Recently, the 4.1 protein, ezrin, radixin and moesin (FERM)-domain–containing kindlin family of proteins has emerged as key players involved in integrin activation. Kindlins cooperate with talin to positively regulate integrin activation. Talin binds the membrane proximal NPxY motif, whereas kindlin binds the membrane distal NxxY motif. Here, we report the crystal structure of human full-length kindlin-3.

Unexpectedly, we observed 3 molecules of kindlin-3 forming a homotrimer in an asymmetric unit of the crystal with each protomer dovetailing the next. Kindlin-3 trimer adopts a triangular prism-like structure along the noncrystallographic 3-fold symmetry axis with the following dimensions: an outer-side length of approximately 110 Å, an inner cavity width of approximately 60 Å, and a height of approximately 90 Å. Each kindlin-3 monomer adopts a cloverleaf-like overall conformation. The F1 domain resides at the center of the kindlin-3 structure with the F1 loop wrapped around its α/β barrel and interacting with other domains. The crystal structure of kindlin-3 trimer also reveals that the additional α2PH helix in the PH domain of protomer A directly wedges into a cleft involving the 2 C-terminal helices (α1F3 and α2F3) and the β-sheet (β5F3-β7F3) in the F3 domain of protomer B, thereby forming extensive contacts. The residues Thr467, Ser468, Val470, Gln471, Ala475, and Ser478 in α2PH of protomer A interact with Ser595, Gln599, Trp600, Ser642, Thr643, Leu656, and Gln659 located in β5F3′ and its preceding loop, and α1F3′ of F3 domain in protomer B (the prime ′ refers to protomer B in the trimer), respectively. In addition, the C-terminus of α1PH and its subsequent loop in the PH domain pack against the 2 C-terminal helices and their connecting loop in the F3 domain of protomer B, through H-bonding (Gln443 in protomer A with main chain of Phe640 in protomer B) and salt bridge (Arg447 in A-Asp653 in B) interactions. In the kindlin-3 trimer, the F3-integrin-binding site in each protomer is occluded by the α2PH helix of the PH domain from the neighboring protomer, suggesting that trimer formation could inhibit kindlin-3 binding to integrin β cytoplasmic tails. Although kindlin-3 monomer binds, albeit weakly with the dissociation constant (Kd) of approximately 200 μM, with integrin β1 cytoplasmic tail, kindlin-3 trimer does not show any detectable binding. Therefore, we proposed that the triple mutations Q471A, A475F, and S478A (henceforth referred to as AFA) could disrupt the protomer–protomer interface in kindlin-3 trimer.

>MAGMKTASGDYIDSSWELRVFVGEEDPEAESVTLRVTGESHIGGVLLKIVEQINRKQDWSDHAIWWEQKRQWLLQTHWTLDKYGILADARLFFGPQHRPVILRLPNRRALRLRASFSQPLFQAVAAICRLLSIRHPEELSLLRAPEKKEKKKKEKEPEEELYDLSKVVLAGGVAPALFRGMPAHFSDSAQTEACYHMLSRPQPPPDPLLLQRLPRPSSLSDKTQLHSRWLDSSRCLMQQGIKAGDALWLRFKYYSFFDLDPKTDPVRLTQLYEQARWDLLLEEIDCTEEEMMVFAALQYHINKLSQSGXXXXXXXXXXXXXXXXXXXXXXXXXXXXXXXXXXXXXXXXXPELKDHLRIFRIPRRPRKLTLKGYRQHWVVFKETTLSYYKSQDEAPGDPIQQLNLKGCEVVPDVNVSGQKFCIKLLVPSPEGMSEIYLRCQDEQQYARWMAGCRLASKGRTMADSSYTSEVQAILAFLSLQRTGSGGPGNHPHGPDASAEGLNPYGLVAPRFQRKFKAKQLTPRILEAHQNVAQLSLAEAQLRFIQAWQSLPDFGISYVMVRFKGSRKDEILGIANNRLIRIDLAVGDVVKTWRFSNMRQWNVNWDIRQVAIEFDEHINVAFSCVSASCRIVHEYIGGYIFLSTRERARGEELDEDLFLQLTGGHEAFLEHHHHHH[3x]> MKITAIHLYAIRLPLRNPFVISYGSYSDMPSIIVKMETDEGIIGYGEGVADDHVTGESWESTFHTLKHTLTPALIGQNPMNIEKIHDMMDNTIYGVPTAKAAIDIACFDIMGKKLNQPVYQLIGGRYHEEFPVTHVLSIADPENMAEEAASMIQKGYQSFKMKVGTNVKEDVKRIEAVRERVGNDIAIRVDVNQGWKNSANTLTALRSLGHLNIDWIEQPVIADDIDAMAHIRSKTDLPLMIDEGLKSSREMRQIIKLEAADKVNIKLMKCGGIYPAVKLAHQAEMAGIECQVGSMVESSVASSAGFHVAFSKKIITSVELTGPLKFTKDIGNLHYDVPF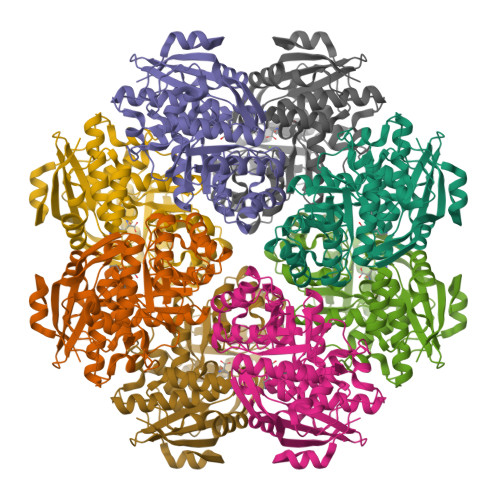IRLNEKPGLGIEINEDTLQELTVFQDIVR> MSGLPPPPPGFEEDSDLALPPPPPPPPGYEIEELDNPMVPSSVNEDTFLPPPPPPPSNFEINAEEIVDFTLPPPPPPPGLDELETKAEKKVELHGKRKLDIGKDTFVTRKSRKRAKKMTKKAKRSNLYTPKAEMPPEHLRKIINTHSDMASKMY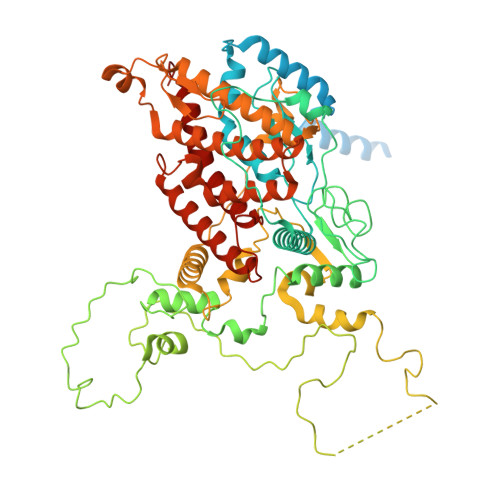NTDKKAFLGALKYLPHAILKLLENMPHPWEQAKEVKVLYHTSGAITFVNETPRVIEPVYTAQWSATWIAMRREKRDRTHFKRMRFPPFDDDEPPLSYEQHIENIEPLDPINLPLDSQDDEYVKDWLYDSRPLEEDSKKVNGTSYKKWSFDLPEMSNLYRLSTPLRDEVTDKNYYYLFDKKSFFNGKALNNAIPGGPKFEPLYPREEEEDYNEFNSIDRVIFRVPIRSEYKVAFPHLYNSRPRSVRIPWYNNPVSCIIQNDEEYDTPALFFDPSLNPIPHFIDNNSSLNVSNTKENGDFTLPEDFAPLLAEEEELILPNTKDAMSLYHSPFPFNRTKGKMVRAQDVALAKKWFLQHPDEEYPVKVKVSYQKLLKNYVLNELHPTLPTNHNKTKLLKSLKNTKYFQQTTIDWVEAGLQLCRQGHNMLNLLIHRKGLTYLHLDYNFNLKPTKTLTTKERKKSRLGNSFHLMRELLKMMKLIVDTHVQFRLGNVDAFQLADGIHYILNHIGQLTGIYRYKYKVMHQIRACKDLKHIIYYKFNKNLGKGPGCGFWQPAWRVWLNFLRGTIPLLERYIGNLITRQFE> SMSAGPWKMVVWDEDGFQGRRHEFTAECPSVLELGFETVRSLKVLSGAWVGFEHAGFQGQQYILERGEYPSWDAWGGNTAYPAERLTSFRPAACANHRDSRLT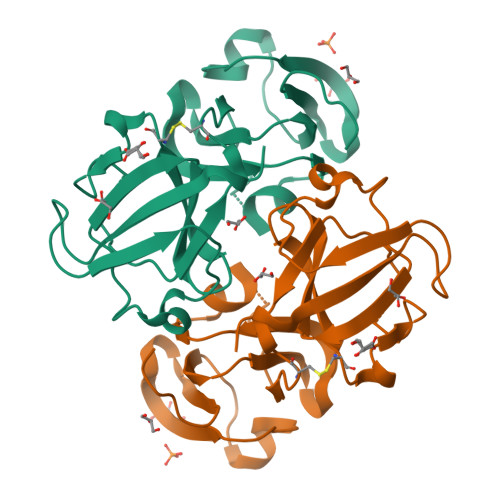IFEQENFLGKKGELSDDYPSLQAMGWEGNEVGSFHVHSGAWVCSQFPGYRGFQYVLECDHHSGDYKHFREWGSHAPTFQVQSIRRIQQ> CNIKNGRCEQFCKNSADNKVVCSCTEGYRLAENQKSCEPAVPFPCGRVSVSQTSKLTR;> IVGGEDAKPGQFPWQVVLNGKVDAFCGGSIVNEKWIVTAAHCVETGVKITVVAGEHNIEETEHTEQKRNVIRIIPHHNYNAAINTYNHDIALLELDEPLVLNSYVTPICIADKEYTNIFLKFGSGYVSGWGRVFHKGRSALVLQYLRVPLVDRATCLRSTKFTITNNMFCAGFHEGGRDSCQGDS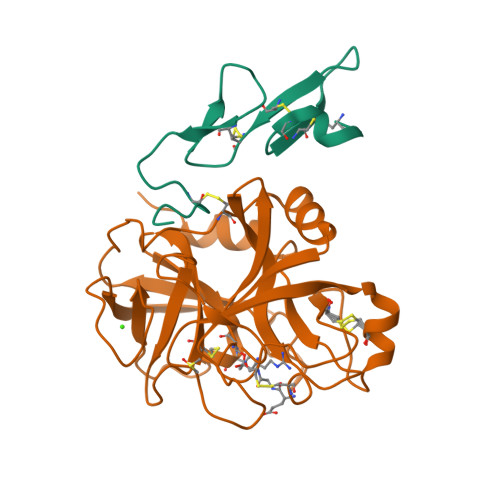GGPHVTEVEGTSFLTGIVSWGEECAMKGKYGIYTKVSRYVNWIKEKTKLT Particularly striking is the much larger size (~260 amino acids) of their single capsid or core proteins (CPs) which in mammalian HBVs comprise only ~180 aa. DHBV CP (DHBc) expressed in E. coli self-assembles into CLPs which package bacterial RNA. In line with earlier data the major type of DHBc CLP conformed to the clustered-dimer T = 4 architecture known from HBc. Confirming selective aspects of evolutionary conservation between avi- and orthohepadnaviruses, the new data also reveal unique structural modules, including a direct contribution of the very C-terminal residues to the capsid shell and a centrally inserted extension of ~45 aa that behaves like an independent folding entity.

The low folding propensity of the extension domain questioned a direct role in capsid assembly. We therefore replaced residues 78–122 by a short G2SG2 linker and evaluated the consequences on assembly and particle morphology. The corresponding protein, DHBc_Δ78–122, was virtually insoluble; however, solubility was drastically improved by the additional mutation R124E (DHBcR124EΔ). Sedimentation, NAGE and negative staining EM data all indicated the formation of orderly CLPs, prompting a closer look by cryo-EM image reconstruction. The resulting density maps at 3 Å resolution (Figure 1—figure supplements 4 and 5) revealed the same architecture as in the wt DHBc particles, except that all spikes remained narrow as also confirmed by the asymmetric analysis. Also, the fold of the subunits in the asymmetric unit was nearly superimposable on that of the full length protein subunits with an RMSD of 0.6 Å, except for the missing sideward pointing density. This missing density was accounted for by the 45 amino acids of the deleted extension domain whereas the flexible G2SG2 linker was not resolved. Difference mapping confirmed that all density differences between full length and internal deletion variant localized to the extension domain which therefore behaves much like an independent internal appendix. Notably, this helical framework forms independently of the extension domain. Of the extension-less variants only Δ78–122_R124E produced specific though weak signals.

>MDINASRALANVYDLPDDFFPKIDDLVRDAKDALEPYWKSDSIKKHVLIATHFVDLIEDFWQTTQGMHEIAESLRAVGGSGGAEIHAHLKAYAKINEESLDRARRLLWWHYNCLLWGEAQVTNYISRLRTWLSTPEKYRGRDAPTIEAITRPIQVAQGGRKTTTGTRKPRGLEPRRRKVKTTVVYGRRRSKSRERRAPTPQRAGSPLPRSSSSHHRSPSPRK[6x]>[6x]MNDKKIELLTTYLSLYIDHHTVLADMQNATGKYVVLDVRNAPAQVKKDQIKGAIAMPAKDLATRIGELDPAKTYVVYDWTGGTTLGKTALLVLLSAGFEAYELAGALEGWKG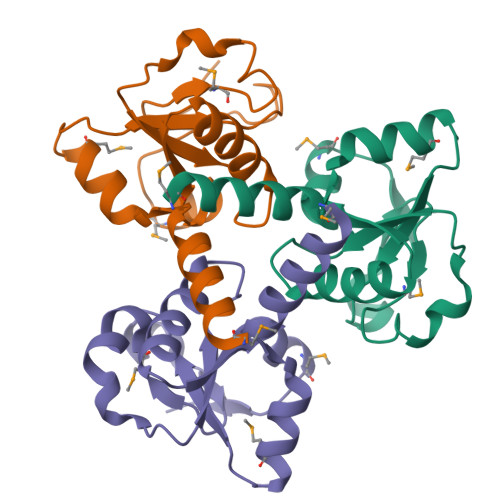MQLPVETLADLEHHHHHH> MALSTIVSQRKQIKRKAPRGFLKRVFKRKKPQLRLEKSGDLLVHLNCLLFVHRLAEESRTNACASKC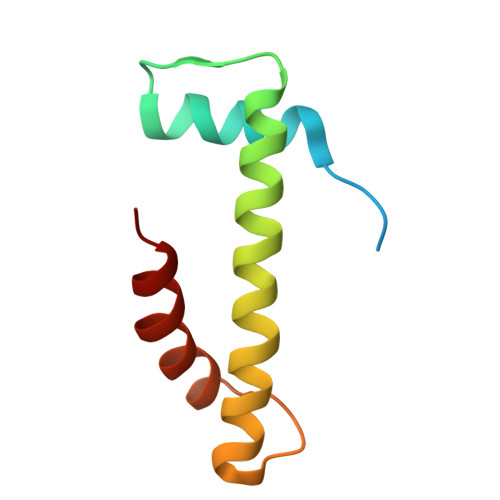RVINKEHVLAAAKVILKKSRG> GMTLRAAVFDLDGVLALPAVFGVLGRTEEALALPRGLLNDAFQKGGPEGATTRLMKGEITLSQWIPLMEENCRKCSETAKVCLPKNFSIKEIFDKAISARKINRPMLQAALMLRKKGFTTAILTNTWLDDRAERDGLAQLMCELKMHFDFLIESCQVGMVKPEPQIYKFLLDTLKASPSEVVFLDDIGANLKPARDLGMVTILVQDTDTALKELEKVTGIQLLNTPAPLPTSCNPSDMSHGYVTVKPRVRLHFVELG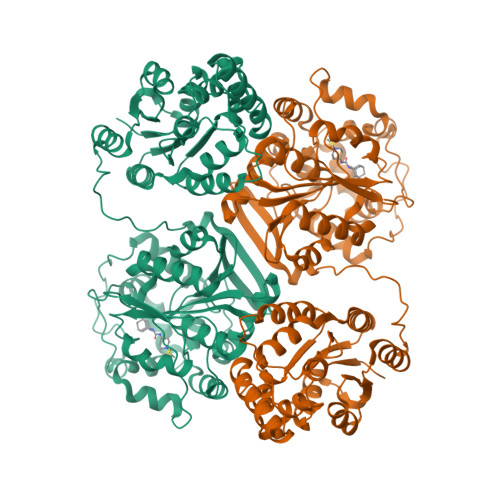SGPAVCLCHGFPESWYSWRYQIPALAQAGYRVLAMDMKGYGESSAPPEIEEYCMEVLCKEMVTFLDKLGLSQAVFIGHDWGGMLVWYMALFYPERVRAVASLNTPFIPANPNMSPLESIKANPVFDYQLYFQEPGVAEAELEQNLSRTFKSLFRASDESVLSMHKVCEAGGLFVNSPEEPSLSRMVTEEEIQFYVQQFKKSGFRGPLNWYRNMERNWKWACKSLGRKILIPALMVTAEKDFVLVPQMSQHMEDWIPHLKRGHIEDCGHWTQMDKPTEVNQILIKWLDSDARN>[4x]GSH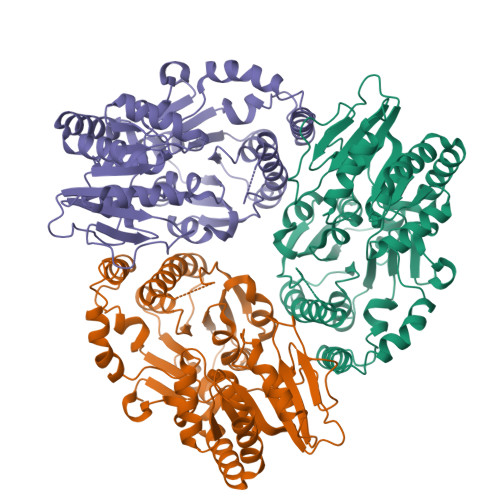MPRPGHIAMVSVPSRGHLHPSLELIRELVARGHRVTYANDPSVAAAVTETGAELVPYTSALPSTDTTEGRVTDQIAQMDVFLDDAVGMLPQLRAAYEEDRPDVFLYDVLAYPARVLAMNWGIPSIQISPTWVMPEKYRERMAPVVEQLKQDPRGAAHYRRFDAWLEDSGVPGIDAGDLVNLPERSLVLVPRFLQPDADDVDEKRFTFIGPCLGRRAHQGDWKRPAGAEKVALVSLGSHLTNQLPFYETCVEVFAALPDWHLVLQIGRHVDAGELGELPPNVEVHNWVPQLAVLEQADVFVTHGGMGGIQEGLFSGVPMVVAPQANDQPANAESVVGLGIARRIDIATVTPDRLRAAVVELASDPAVAERLSGLRRELRAHGGTMRAADLIERQLPA3-selanylpropanoic acid | C3 H6 O2 Se | 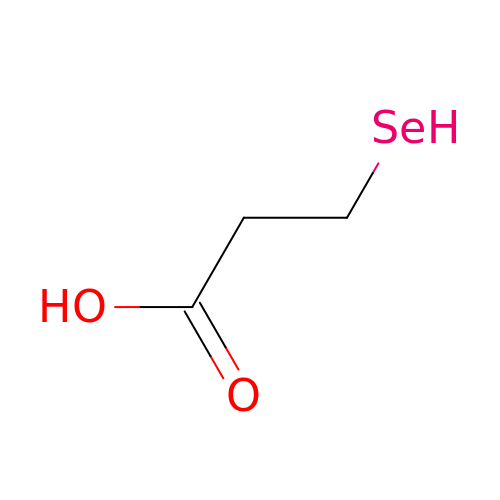DGRAMMLRUJGIJS-UHFFFAOYSA-N> MANLYVKAVPPPDMNRNTEWFMYPGVWTT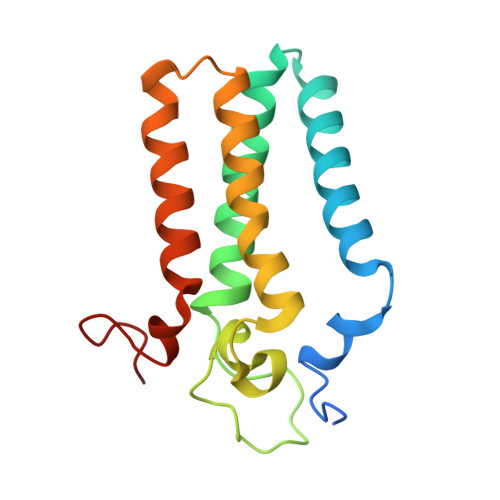YMLILFFGWLVVLSVSGCSPGMAWTVVNLAHFVVTYHSFHWMKGTPFADDQGIYNGLTWWEQMDNGQQLTRNRKFLTLVPVVLYLIASHTTDYRHPWLFLNTLAVMVLVVAKFPNMHKVRIFGINGDK> XSLSSKQKATVKDFFSKMSTRSDDIGA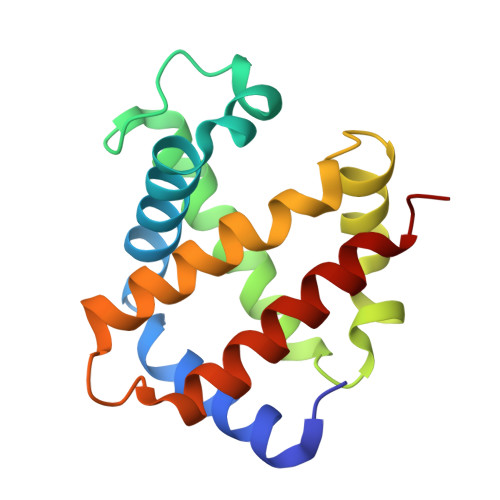EALSRLVAVYPQTKSYFSHWKDASPGSAPVRKHGITIMGGVYDAVGKIDDLKGGLLSLSELHAFMLRVDPVNFKLLAHCMLVCMSMIFPEEFTPQVHVAVDKFLAQLALALAEKYR>[2x]GPHMLGILNKMFDPTKRTLNRYEKIANDIDAIRGDYENLSDDALKHKTIEFKERLEKGATTDDLLVEAFAVVREASRRVTGMFPFKVQLMGGVALHDGNIAEMKTGEGKTLTSTLPVYLNALTGKGVHVVTVNEYLASRDAEQMGKIFEFLGLTVGLNLNSMSKDEKREAYAADITYSTNNELGFDYLRDNMVLYKEQMVQRPLHFAVIDEVDSILIDEARTPLIISGQAAKSTKLYVQANAFVRTLKAEKDYTYDIKTKAVQLTEEGMTKAEKAFGIDNLFDVKHVALNHHINQALKAHVAMQKDVDYVVEDGQVVIVDSFTGRLMKGRRYSEGLHQAIEAKEGLEIQNESMTLATITFQNYFRMYEKLAGMTGTAKTEEEEFRNIYNMQVVTIPTNRPVVRDDRPDLIYRTMEGKFKAVAEDVAQRYMTGQPVLVGTVAVETSELISKLLKNKGIPHQVLNAKNHEREAQIIEEAGQKGAV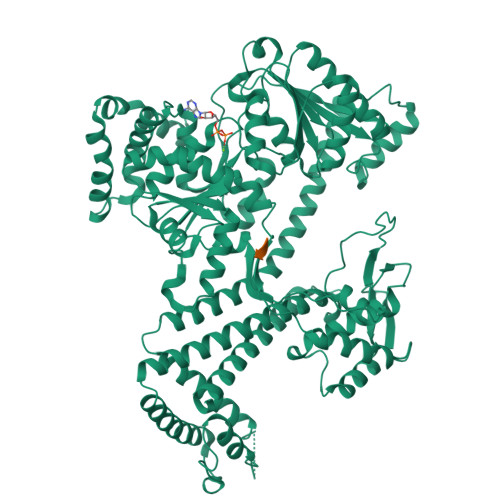TIATNMAGRGTDIKLGEGVKELGGLAVVGTERHESRRIDNQLRGRSGRQGDPGITQFYLSMEDELMRRFGAERTMAMLDRFGMDDSTPIQSKMVSRAVESSQKRVEGNNFDSRKQLLQYDDVLRQQREVIYKQRFEVIDSENLREIVENMIKSSLERAIAAYTPREELPEEWKLDGLVDLINTTYLDEGALEKSDIFGKEPDEMLELIMDRIITKYNEKEEQFGKEQMREFEKVIVLRAVDSKWMDHIDAMDQLRQGIHLRAYAQTNPLREYQMEGFAMFEHMIESIEDEVAKFVMKAEI> SNAVVEDSMKATSAEDLSNSIANQNPRGRGGDEDEELEEGEIVGDDDLDSSNLSASLVHQPHPLEHSWTFWFDNPSAKSKQATWGASIRPIYTFSTVEEFW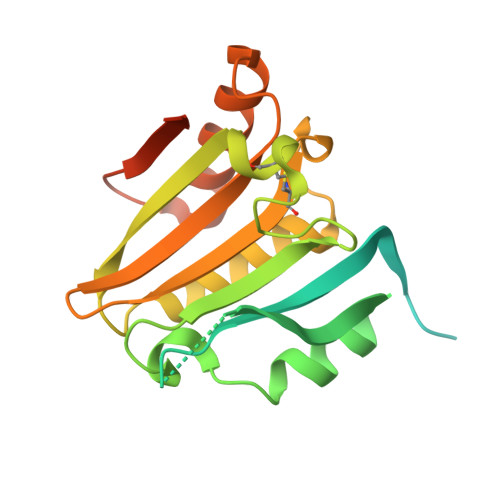SVYNNIHHPSKLAMRADLYCFKHKIEPKWEDPVCANGGKWTVNFPRGKSDNGWLYTLLAMIGEQFDCGDEICGAVVNVRSGQDKISIWTKNASNEAAQASIGKQWKEFLDYNESIGFIFHDDAKKFDRHAKNKYMV>HHHHHHSSGLVPRGSHMQTTTVYSLEDLLPYLKQDNVDVKLAPGTYNVNGFDVGEDRLFSTTPLFLFEGSNSTYDFTDVKLNINTVVLTKFGNNEVNEIQILGNNNVLKNLKLEDIGTTAPSNRAQSIVIDGRDNRIEGFHLTIRGSYPYGYGAAFGKGGGSVINHRKHSGVLIRGLRNHLKDCTIISRSYGHIVFMQAASYPTVEGCYIEGEMRS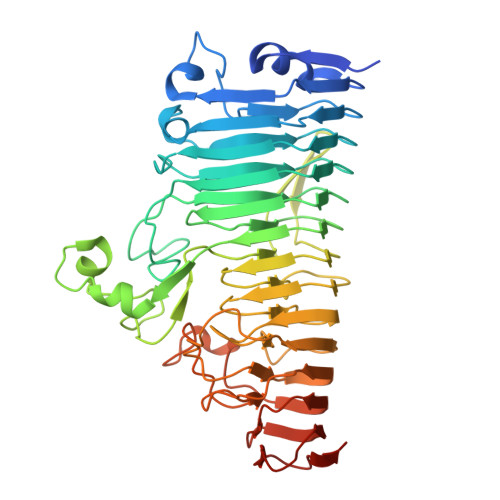TDDMLAEEGTGSPADKVDFMTVWGYKLPAGYMMSLQEGGIRAYNAGTTYIDGVEIQRATDNPTVLNCTIKNARTGVTLAHANGTKYVEGCTVLGCENGYSIGSGTVVNCGADAIYGPVFKNTYGSDKGYNADITILPPSDAYYNGHDAVAYIGGSNHNLTFRSEITEIPSNLKIMVSGDLQGLRVLHGSNPSQNNFAGTNIVLRNLTNFPVDLHSDSSNITVTSCDTDNITDNGTNNSIEAIDCDSD[2x]>[4x]MTRAINDPGNEDPGSLLETDADALLGGAAAQAPEERCRLAAQACIRACERYLALCTESSREQRQHAGDCADLCRLAALLMERRSPWAPAACELAARYALACAERCD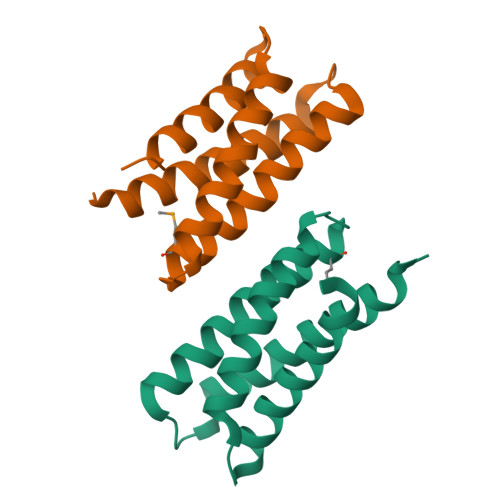GDEPLERECAGACRRFVEACRPLLPALEHHHHHH(2~{R})-3-bis[2-methyl-5-(trifluoromethyl)pyrazol-3-yl]boranyloxypropane-1,2-diol | C13 H15 B F6 N4 O3 | 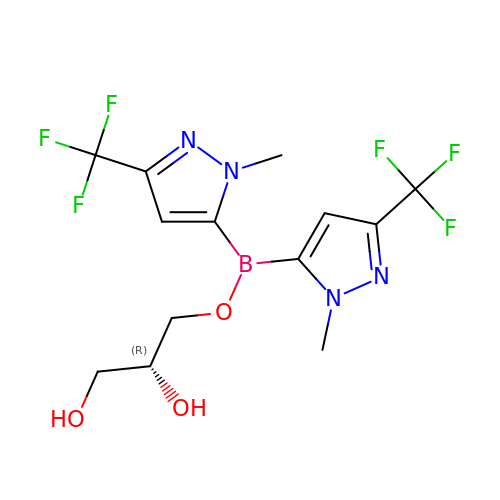ZMDZOWFKTCAOKY-SSDOTTSWSA-N>MAHHHHHHMSVIQDLQSRGLIAQTTDIEALDALLNEQKIALYCGFDPTADSLHIGHLLPVLALRRFQQAGHTPIALVGGATGMIGDPSFKAAERSLNSAETVAGWVGSIRSQLTPFLSFEGGNAAIMANNADWFGSMNCLDFLRDIGKHFSVNAMLNKESVKQRIDRDGAGISFTEFAYSLLQGYDFAELNKRHGAVLEIGGSDQWGNITAGIDLTRRLNQKQVFGLTLPLVTKSDGTKFGKTEGGAVWLNAKKTSPYQFYQFWLKVAD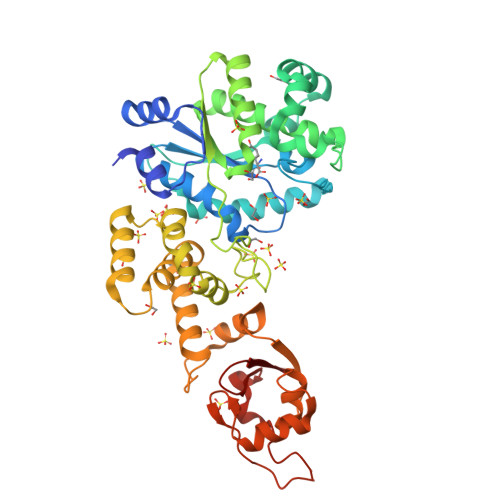ADVYKFLKYFTFLSIEEIGVVEAKDKASGSKPEAQRILAEEMTRLIHGEEALAAAQRISESLFAEDQSRLTESDFEQLALDGLPAFEVSDGINAVEALVKTGLAASNKEARGFVNAKAVLLNGKPAEANNPNHAAERPDDAYLLIGEYKRFGKYTILRRGKRNHALLVWK[2x]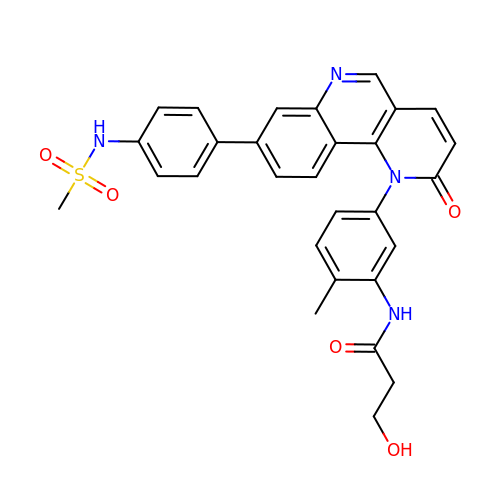~{N}-[2-methyl-5-[8-[4-(methylsulfonylamino)phenyl]-2-oxidanylidene-benzo[h][1,6]naphthyridin-1-yl]phenyl]-3-oxidanyl-propanamide | C29 H26 N4 O5 S | PBOKXQRUWSFTHG-UHFFFAOYSA-N> MSANKAIINIDQELCTGCRRCAEVCPVDAIEGEKGKPQKINTEVCVMCGQCVQKCSSYASYFDESITPRNVKLQERGMLDSVKEPLFAAYNLGYARQVKEALENPQLFKVVQCAPAIRVSIAEEFGLDLGDLTPGKLVAALRRLNFDRVYDTNFGADLTIIEEANELVKRIKEGKDLPMFTSCCPAWVKFAEQTYPELLKHISTCKSPQQMTG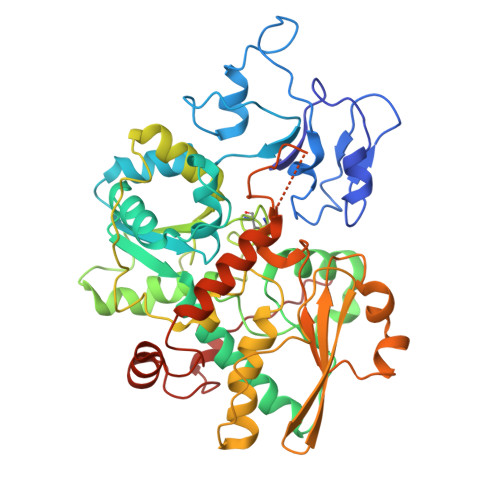AIIKTYGAKINNVDPAKIFSVSVMPCTCKSYESDRPEMRSSGYKDVDLVITTRELAHLMKDKGIDFATLPDEEFDSPLGNYTGAATIFGNTGGVMEAALRTAYELITKKPIPNIDIEFVRGGEGIRTATVQVGELELKIAVVSGLKNVIPILEDIKKNKCDLHFVEVMTCPEGCISGGGQPKLLLEEYREVAYKKRKEALYKHDAELELRKSHENPAIKKLYEEFLGEPLGKQSHHLLHTKYTPRKKV>[4x]GPGSMFDLQGRSVVVTGGTKGIGRGIATVFARAGANVAVAGRSTA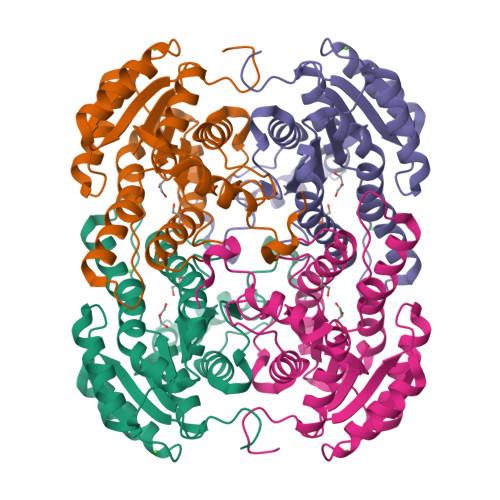DIDACVADLDQLGSGKVIGVQTDVSDRAQCDALAGRAVEEFGGIDVVCANAGVFPDAPLATMTPEQLNGIFAVNVNGTFYAVQACLDALIASGSGRVVLTSSITGPITGYPGWSHYGATKAAQLGFMRTAAIELAPHKITVNAIMPGNIMTEGLLENGEEYIASMARSIPAGALGTPEDIGHLAAFLATKEAGYITGQAIAVDGGQVLPESLDAIAT N-[(4aS,6S,8aR)-2-amino-5,6,7,8-tetrahydro-4a,8a-(methanooxymethano)-3,1-benzothiazin-6(4H)-yl]-3-chlorobenzamide 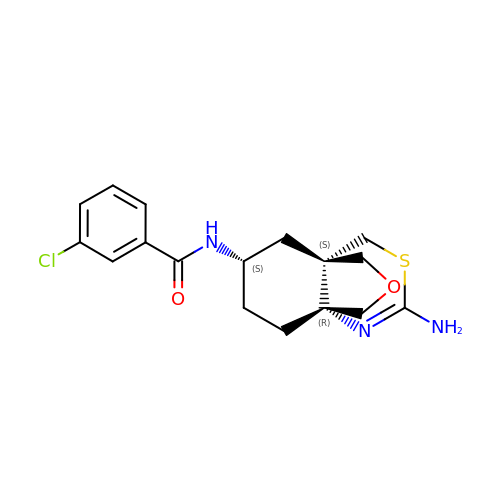| C17 H20 Cl N3 O2 S | XDMHBNONUZHFDP-JQFCIGGWSA-N> LTTSLEQDPDEQDANREIAAATKQTVETLMAGERIAEALELGMTDLNTIREWEEARQINPNIAPPQRNPIFVALGNIPAETYVLNTLQKIK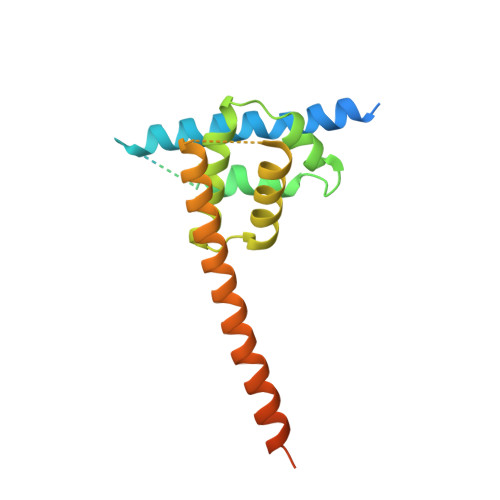PASLHDALLVLPFSTIPSLLTFLNLFAQRELNVPLTCRILFFVLKTHHKQIVASRTMRATLEKVRANLRAALRRQKDEMGFNIAALKVVSMQLRDKSVREYVDETWEEKEKEKGVRKR> GHMSHLADVSPPTACRVCGGGVQEFLDLGRQPLSDRFRKPDELDDEFTYRLAVGRCDSCEM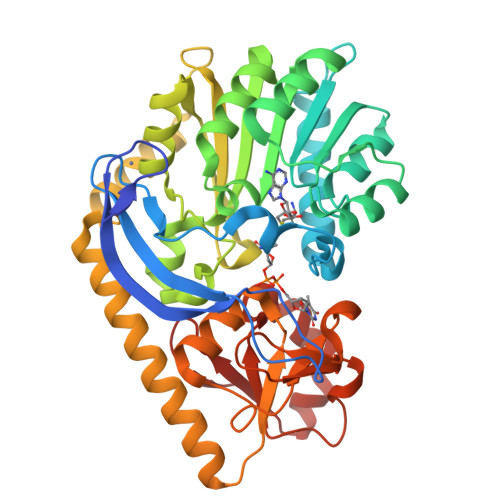VQLTEEVPRDLMFHEVYPYHSSGSSVMREHFAMLARDFLATELTGPDPFIVEIGCNDGIMLRTIQEAGVRHLGFEPSSGVAAKAREKGIRVRTDFFEKATADDVRRTEGPANVIYAANTLCHIPYVQSVLEGVDALLAPDGVFVFEDPYLGDIVAKTSFDQIYDQHFFLFSATSVQGMAQRCGFELVDVQRLPVHGGEVRYTLARQGSRTPSAAVAQLLAAEREQELSDMATLRAFAGNVVKIRDELTALLHRLRAEGRSVVGYGATAKSATVTNFCGIGPDLVHSVYDTTPDKQNRLTPGAHIPVRPASAFSDPYPDYALLFAWNHAEEIMAKEQEFHQAGGRWILYVPEVHIR> IVGGTNSSWGEWPWQVSLQVKLTAQRHLCGGSLIGHQWVLTAAHCFDGLPLQDVWRIYSGILNLSDITKDTPFSQIKEIIIHQNYKVSEGNHDIALIKLQAP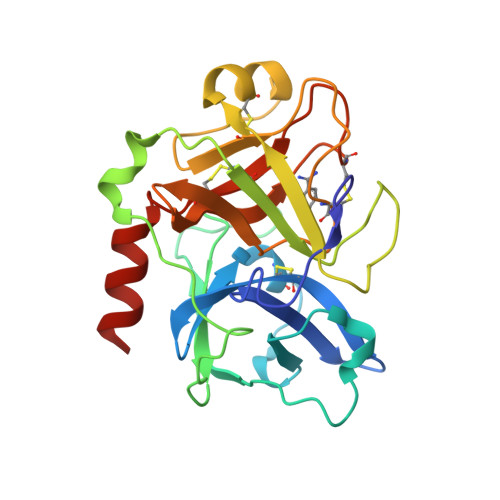LNYTEFQKPISLPSKGDTSTIYTNCWVTGWGFSKEKGEIQNILQKVNIPLVTNEECQKRYQDYKITQRMVCAGYKEGGKDACKGDSGGPLVCKHNGMWRLVGITSWGEGCARREQPGVYTKVAEYMDWILEKTQSSDGK> ANFNVPKLGVFPVAAVFDIDNVPEDSSATGSRWLPSIYQGGNYWGGGPQALHAQVSNFDSSNRLPYNPRTENNPAGNCAFAFNPFGQYISNISSAQSVHRRIYGIDLNDEPLFSPNAASITNGGNPTMSQDTGYHNIGPINTAYKAEIFRPVNPLPMSDTAPDPETLEPGQTEPLIKSDGVYSNSGIASFIFDRPVTEPNPNWPPLPPPVIPIIYPTPALGIGAAAAYGFGYQVTVYRWEEIPVEFIADPETCPAQPTTDKVIIRTTDLNPEGSPCAY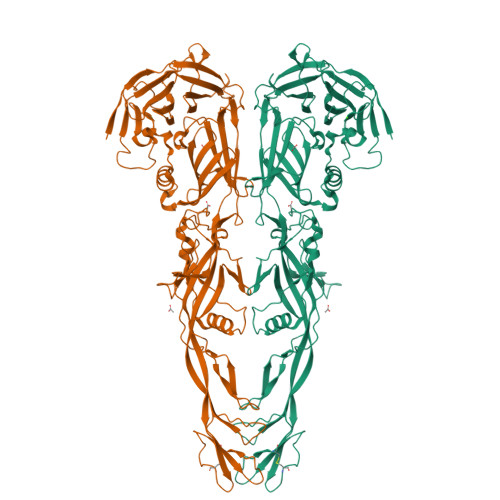EAGIILVRQTSNPMNAVAGRLVPYVEDIAVDIFLTGKFFTLNPPLRITNNYFADDEVKENTVTIGNYTTTLSSAYYAVYKTDGYGGATCFIASGGAGISALVQLQDNSVLDVLYYSLPLSLGGSKAAIDEWVANNCGLFPMSGGLDKTTLLEIPRRQLEAINPQDGPGQYDLFILDDSGAYASFSSFIGYPEAAYYVAGAATFMDVENPDEIIFILRNGAGWYACEIGDALKIADDEFDSVDYFAYRGGVMFIGSARYTEGGDPLPIKYRAIIPGL> AHHHHHHGSGLFDFLKRKEVKEEEKIEILSKKPAGKVVVEEVVNIMGKD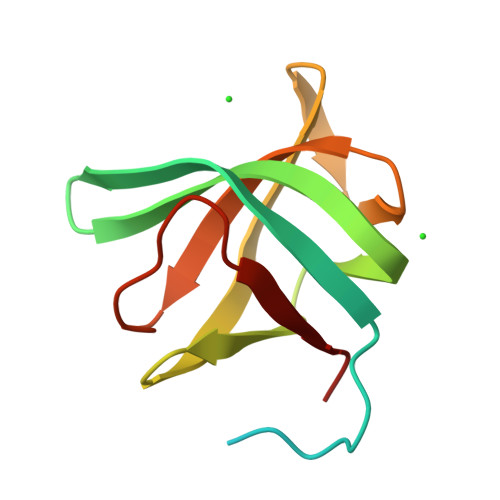VIIGTVESGMIGVGFKVKGPSGIGGIVRIERNREKVEFAIAGDRIGISIEGKIGKVKKGDVLEIYQT>[8x]GHMSTLLINQPQYAWLKELGLREENEGVYNGSWGGRGEVITTYCPANNEPIARVRQASVADYEETVKKAREAWKIWADIPAPKRGEIVRQIGDALREKIQVLGSLVSLEMGKILVEGVGEVQEYVDICDYAVGLSRMIGGPILPSERSGHALIEQWNPVGLVGIITAFNFPVAVYGWNNAIAMICGNVCLWKGAPTTSLISVAVTKIIAKVLEDNKLPGAICSLTCGGADIGTAMAKDERVNLLSFTGSTQVGKQVGL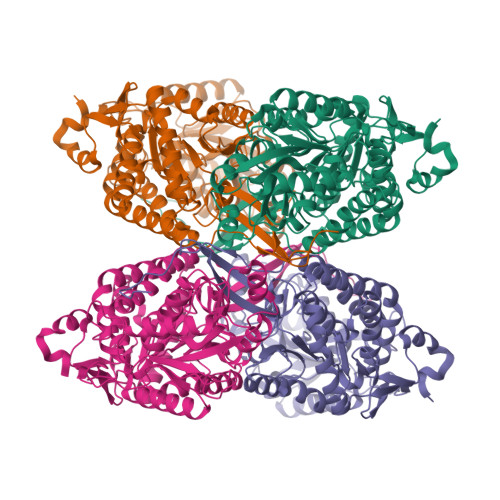MVQERFGRSLLELGGNNAIIAFEDADLSLVVPSALFAAVGTAGQRCTTARRLFIHESIHDEVVNRLKKAYAQIRVGNPWDPNVLYGPLHTKQAVSMFLGAVEEAKKEGGTVVYGGKVMDRPGNYVEPTIVTGLGHDASIAHTETFAPILYVFKFKNEEEVFAWNNEVKQGLSSSIFTKDLGRIFRWLGPKGSDCGIVNVNIPTSGAEIGGAFGGEKHTGGGRESGSDAWKQYMRRSTCTINYSKDLPLAQGIKFQ>MVMSQKPITLYVGADYVSAFAMSAFVVLKEKGLDFEIRTVDLKSKQQHGSAYREVSLTRRVPTLQHDRFTLSESSAIAEYLDEVYPAPHYAAVLPADRETRALARQLQAWIRSDFMPLKSERQADRIYFPEPVKPLGEAA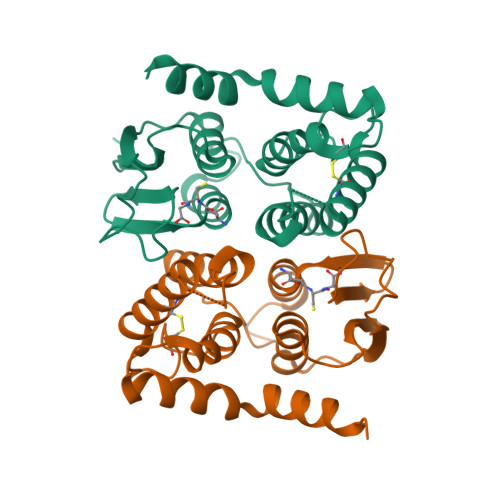QLACEKLLSAADRLIDDERYGVFGDWCIADTDFALMLNRLVACGDPVPPKVLRYVERQWARPSVQQWVKQKRDAENLYFQ[5x]> MAHHHHHHVGTMVEEVDENSWEEKVLKSDKPVVVYFWAPWCGPCE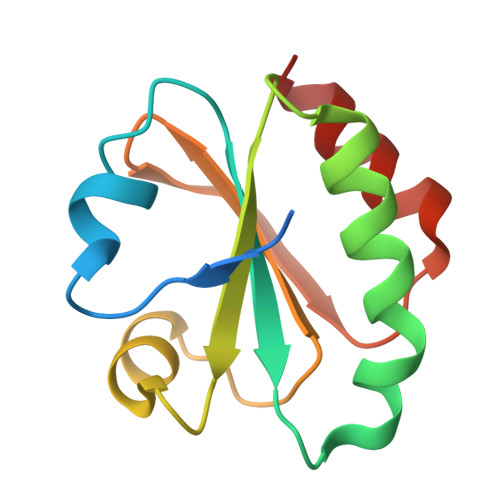EIKPIIEKLAEKYAGKVRVYRVDVDKAPGIAEKYNITSVPAVLIFKDGKLLKKLFGVIPEEELEKWIKEVL>MAHHHHHHSAALEVLFQGPGGHLLGNRYGKIENGKLNIYSLADNSLIKTVEAGPWENMAYSMDSNSINNIDGYISYTGWYRPYGTSQDGKTWYPTTVADWRPILMYVWPSKDVQAKFIQYFVNHGYENSNYGLTTGSVKDLSENTASIKLNEVAQNLRYVIEQHIVAAKSTSQLANDINNFITTIPELSASSELPYGQVIFVNNDNTSYADSKYRLMSRTINNQTGNDNDNSDNGYEFLTGIDIDNSNPVVQAENLNWEYFLLNYGKLMGYNPDGNFDGFRIDAADHIDADVLDQTGQLMDDMYHMKGNPQNANNHLSYNEGYRSSAARMLNKKGNPQLYMDYVGSTLGNVLGRANNRDTISNLVTGSIVNRQNDVTENEATPNWSYVTNHDSRANLINGLISKDHPGAYKAEYANQAWQEFYADQKKTDKQYAQYNVPAQYAILLSNKDTVPQIYYGDLYNETAQYMQEKSIYYDAITTLMKARKQFVSGGQTMTKLSDNLIASVRYGKGVTNANSEGTDSLSRTSGMAVIVGNNP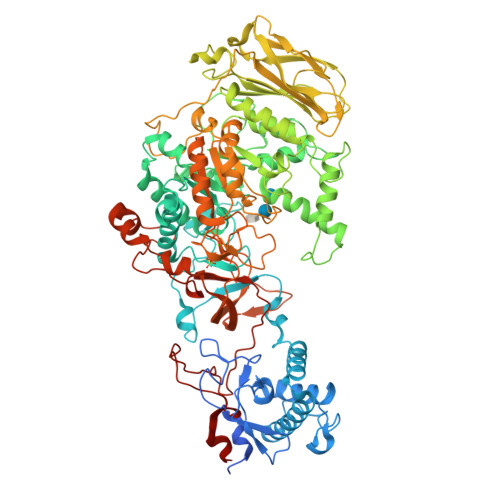QMAEQTISINMGRAHANEQYRNLLDTTDNGLTYNADGAENPETLTTDDNGILKVTVKGYSNPYVSGYLGVWVPVVSGNQDVTTNAATVSADSNKIFESNAALDSHMIYQDFSLYQPEPTSTENHAYNTIAQNAELFNNLGITDFWMAPPYTQYSESRYNDGYSVTDRYNLGTNANPTKYGSGEELANAIAALHSAGLKVQVDIVMNQMIGLPGQEAVTVTRADNRGIQTYVNGKTYANQMYFAYTTGGGNGQETYGGKYLSELQSKYPDLFTTRAISTGVAPDPTTRITKWSAKYENGTSLQNIGIGLAVKLPNGEYAYLRSSDNKAFNTTLPETMSSADYYAN[2x]>[2x]MFKDGSLIPYLTAGDPDKQSTLNFLLALDEYAGAIELGIPFSDPIADGKTIQESHYRALKNGFKLREAFWIVKEFR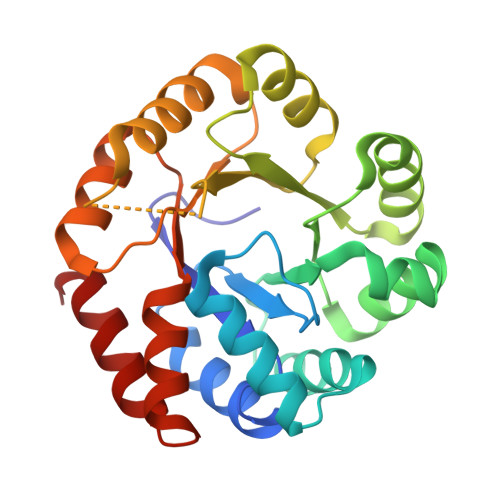RHSSTPIVLMTYYNPIYRAGVRNFLAEAKASGVDGILVVDLPVFHAKEFTEIAREEGIKTVFLAAPNTPDERLKVIDDMTTGFVYLVSLYGTTGAREEIPKTAYDLLRRAKRICRNKVAVGFGVSKREHVVSLLKEGANGVVVGSALVKIIGEKGREATEFLKKKVEELLGI> MGDTTQLVKEYQEKRSKLEKFMKNPQHDASLLSNSNEFRDKNVEFFASGGTRTSKFDKLENHP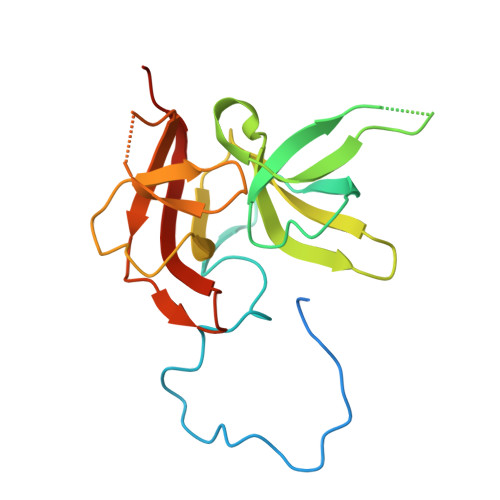FLGYPYKRGVKRVIQEAQDNQSHYEPHVEAGGGEDLYGICIDIDEFSKTATIVPITNNFEGYLVAKDSTVKVKDKLIFNKDGALEKVTGAPNKATINATALTDAKQISNEVYLVKVAVFGNKAMSRN>IVGGYTCGANTVPYQVSLNSGYHFCGGSLINSQWVVSAAHCYKSGIQVRLGEDNINVVEGNEQFISASKSIVHPSYNSETYNNDIMLIKLKSAASLNSRVASISLPTSCASAGTQCLISGWGNTKSSGTSYPDVLKCLKAPILSDSSCKSASSFIITSNMFCVGYLEGGKDACQGDSGGPVVCSGKLQGIVSWGEGCAQKNKP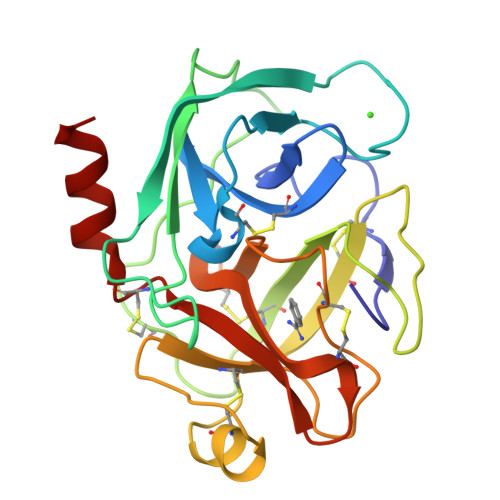GFYTKVCNYVSWIKQTIASN[16x]> MSHHHHHHSMTAKTPLDPALFRPDAISDETRGINDFIIKAFEAVPEWWEIGAATVREARARGEGGFPLPPKSERARTIEIEGKGGHKVPLRIIAPESPKGVYLHIHGGGWVLGACDQQDPMLERIAQNAGLACVSVEYRLAPEHPYPAGPDDCEA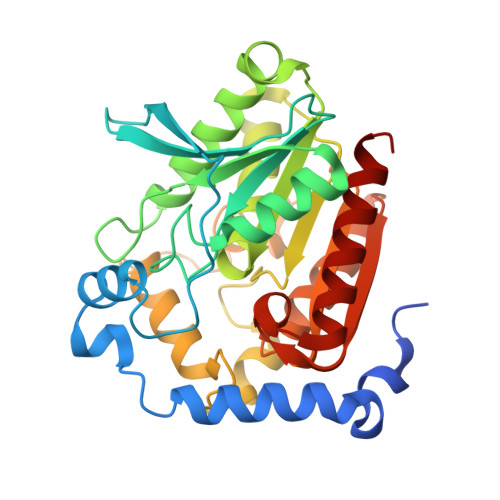AALWLVKNAKKEFGTEVLTIGGESAGGHLSAVTLLRMRDRHGYKGFKGANLVFGAFDMSMSPSQRVFGNERLVLRTVDIQKFGDAFLPNGEDRRDPDISPLYANLHDMPPALFTVGTRDALVDDTLFMHARWIAAGNEAELGVFPGGAHGFVAFPGEIARAANAQADAFLRRVTGQ>[6x]MSFDPLPGTLENLLEQTSLKWIFVGGKGGVGKTTTSCSLAIQMSKVRSSVLLISTDPAHNLSDAFGTKFGKDARKVPGFDNLSAMEIDPNLSIQEMTEQADQQNPNNPLSGMMQDLAFT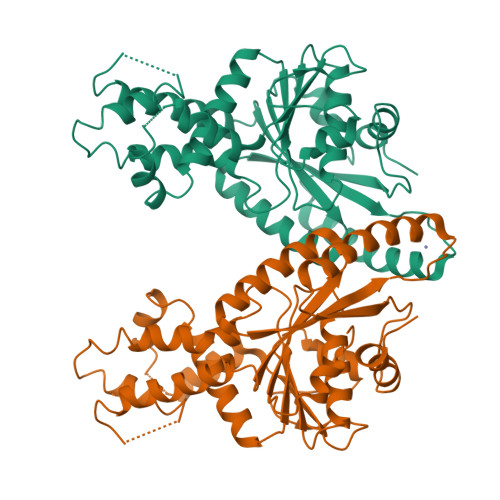IPGIDEALAFAEILKQIKSMEFDCVIFDTAPTGHTLRFLNFPTVLEKALGKLGGLSSRFGPMINQMGSIMGVNANEQDLFGKMESMRANISEVNKQFKNPDLTTFVCVCISEFLSLYETERMIQELTSYEIDTHNIVVNQLLLDPNTTCPQCMARRKMQQKYLAQIEELYEDFHVVKVPQVPAEVRGTEALKSFSEMLVKPYVYPTSGKE> MSAPPNTLFLRLEGALQSWGSNEAKFALRRTADAPTKSGVLGLLCAAMGIGRAEAADSWLPKLANLRMGVRIDRPGIRWWDFHTVGAGQRMRMAELKAPKKPSMVGAALAETLTPSKVKTRAETLLSRREYLADASFLVALQGEPELVAKLSAALAKPVWAIYLGRKSCPPSRPVCEHPPGFYN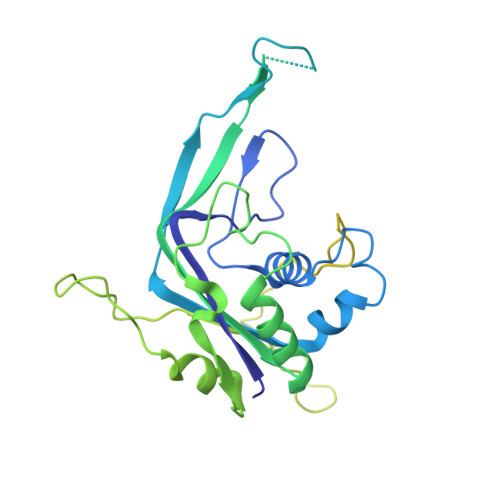TLEEALSAVPLQKRWHNEPLPQILPCVMDWIPGYDGEHAPDDAEIHYDLPVSFQPPRHLPRFVIRRELVVGEDVQVSRETGTSVWRPKGTRADYNNSEYKKVRAERLVMDHAACMVCKAPATTVQHVNYRRAGGKEIPEDLRALCRLCHDACTMLEYGSGMTTNRIDPCDPIWRERILAKRKEIVEFRSRGQRFRKMKPEEENG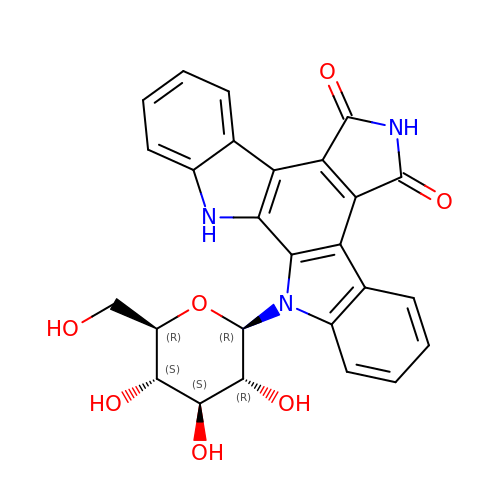12-beta-D-glucopyranosyl-12,13-dihydro-5H-indolo[2,3-a]pyrrolo[3,4-c]carbazole-5,7(6H)-dione | C26 H21 N3 O7 | FAKJOUAYZNXZGV-QCUUGYDUSA-N> MN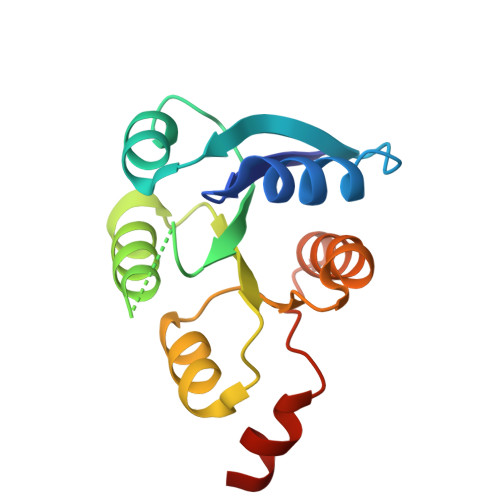NMNVIIADDHPIVLFGIRKSLEQIEWVNVVGEFEDSTALINNLPKLDAHVLITDLSMPGDKYGDGITLIKYIKRHFPSLSIIVLTMNNNPAILSAVLDLDIEGIVLKQGAPTDLPKALAALQKGKKFTPESVSRLLEKISA> S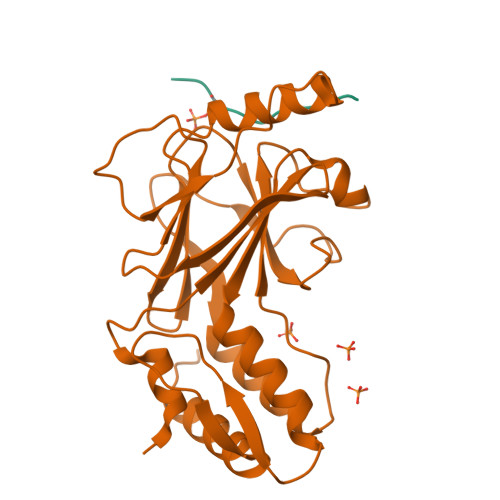EFENPLKRLLVPGEEWEFEVTAFYRGRQVFQQTISCPEGLRLVGSEVGDRTLPGWPVTLPDPGMSLTDRGVMSYVRHVLSCLGGGLALWRAGQWLWAQRLGHCHTYWAVSEELLPNSGHGPDGEVPKDKEGGVFDLGPFIVDLITFTEGSGRSPRYALWFCVGESWPQDQPWTKRLVMVKVVPTCLRALVEMARVGGASSLENTVDLHISNSHPLSLTSDQYKAYLQDLVEGMDFQGPGES;> STLTEEFELLISNSEDDWE> MWPSAKFIDGRVAFSRMPAERELDEVARDFDAVVVLVEDYELPYSLDEWEKRGVEVLHGPIPDFTAPSVEQLLEILRWIEERVREGKKVLIHCMGGLGRSGTVGVAWLMYSRGLSLREALMEVRRKRPGAVETQ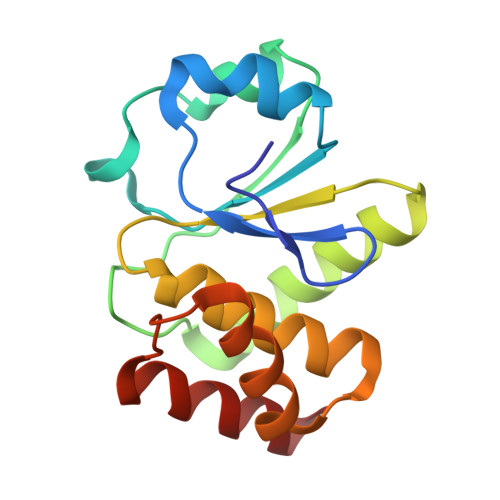EQMEVLKELEERI>[2x]MTSDLIAKLSVNAGEPIGNMRQLHGTSGIPAPAPGTDSVPDILDVWRNAQVTLVRSYDWVSRLDTIDNPTSLFPDWSADPSDPASYNFAATDTWVGQTRSIGANILFTIASEIPANKQPARDLAKYEQVVENIVRHYVCGWGDGFENAVSHWEFGDQPDFGKLHFSGTPDQFYEMYAAAARAVKRVDPALKVGGPCVAFPLNEGPFREGFLDYVKQQSVPLDFLSWMWYGDNSRDPMDFRTIAAEVRAIVDKYGFTDTELLLSYWSMTGIPTAKFEDFDNAAFLAAAAIYMQDSEVDKAIFFRADTGADFHYNFTDPAGIFEDDGSQNARTGAFQLVGQTLATTERLAITGGDDNGFAALAGRTADGDTIRILISNYAIPDMYLTARDRDVFEFQVPIGDQKTDMSLNVPPRRVDARSTGYSGYTLEIGHLPWGDGPHRVVRYRADRDHKGEMLDSHEGRGSSVTVQNKLAVSGVELIEITRVSS

A putative open reading frame of 1458 bp (cmgh1), encoding a protein of 485 aa (CmGH1) with a theoretical molecular weight of 53.48 kDa and pI of 4.66, was identified from the whole-genome of strain C. marinus E4A9T. According to the phylogenetic tree, the protein CmGH1 belongs to the GH39 family. Here, we present the characterizations and crystal structure of CmGH1, which showed β-glucosidase activity, instead of β-xylosidase activity, to provide a structural basis for the development, and utilization of the marine sourced β-glucosidase. Therefore, CmGH1 was evaluated for saccharification potential with different substrates, which turned out that CmGH1 showed β-glucosidase activity when using p-nitrophenyl-β-D-glucopyranoside (p-NPG) and cellobiose as substrates.

The crystal structure of CmGH1 was solved with a 1.8 Å resolution. Diffraction dataset was integrated into the monoclinic space group P21 with two molecules per asymmetric unit. The first four residues at the N-terminal region and the residues from Val396 to Thr403 were invisible in chain A but were refined unambiguously in the electron-density map of chain B. Therefore, we will discuss the Chain B structure only. Structural superimposition showed that CmGH1 shared a similar architecture with other GH39 family β-xylosidases, despite that PslG and GH39wh2 only shared 17% and 13% identities with CmGH1. The groove distances among residues Phe114 and Tyr312, Pro271 and Leu163 of CmGH1 were 6.6 Å and 15.0 Å, respectively, whereas the corresponding distances in the groove of GH39wh2 were 19.3 Å and 22.4 Å (Tyr210 and Glu415, Asn251, and Asn370), and those in XynB were 5.4 Å and 14.6 Å (Tyr116 and Arg324, Tyr282 and Phe166). Therefore, CmGH1 might be a new exoglycosidase when comparing with GH39wh2 and XynB. The active sites of XynB include the conserved Glu160 and nucleophile Glu277, whereas the corresponding residues in CmGH1 were Gln157 and Tyr264. However, Y264E and Q157E/Y264E mutants abolished the enzymatic activities of CmGH1, which suggested that Tyr264 could contribute a vital role in the enzyme activity. For example, the β-hairpin motif of CmGH1 extended from the catalytically active pocket and held onto one end, which was not reported in GH39 family. However, the β-hairpin motif of CmGH1 was far away from the nearby small α-helix, indicating that there was no interaction between them and the β-hairpin motif adopted a closed conformation, which might be related to its substrate recognition.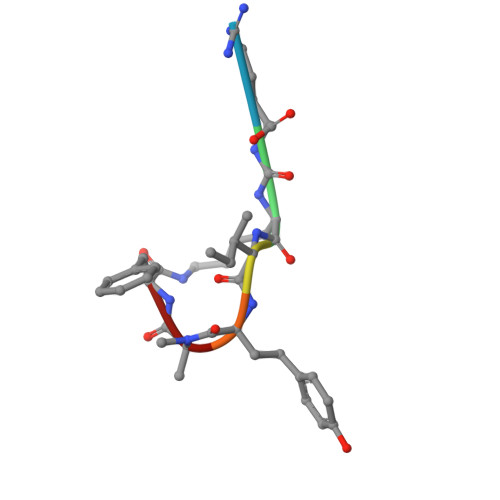> RKIYAF> MELTPREKDKLLLFTAALVAERRLARGLKLNYPESVALISAFIMEGARDGKSVASLMEEGRHVLTREQVMEGVPEMI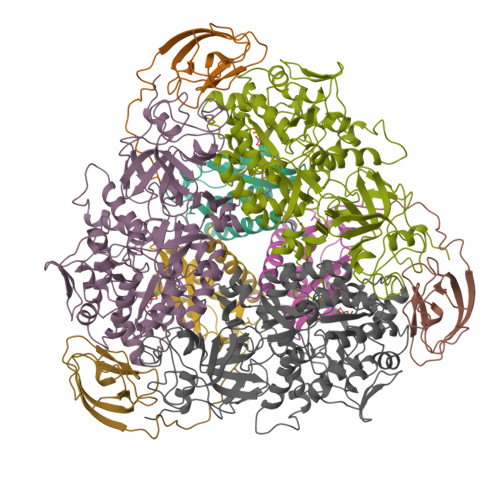PDIQVEATFPDGSKLVTVHNPII;> MIPGEYHVKPGQIALNTGRATCRVVVENHGDRPIQVGSHYHFAEVNPALKFDRQQAAGYRLNIPAGTAVRFEPGQKREVELVAFAGHRAVFGFRGEVMGPLEVNDE;> MSNISRQAYADMFGPTVGDKVRLADTELWIEVEDDLTTYGEEVKFGGGKVIRDGMGQGQMLAADCVDLVLTNALIVDHWGIVKADIGVKDGRIFAIGKAGNPDIQPNVTIPIGAATEVIAAEGKIVTAGGIDTHIHWICPQQAEEALVSGVTTMVGGGTGPAAGTHATTCTPGPWYISRMLQAADSLPVNIGLLGKGNVSQPDALREQVAAGVIGLKIHEDWGATPAAIDCALTVADEMDIQVALHSDTLNESGFVEDTLAAIGGRTIHTFHTEGAGGGHAPDIITACAHPNILPSSTNPTLPYTLNTIDEHLDMLMVAHHLDPDIAEDVAFAESRIRRETIAAEDVLHDLGAFSLTSSDSQAMGRVGEVILRTWQVAHRMKVQRGALAEETGDNDNFRVKRYIAKYTINPALTHGIAHEVGSIEVGKLADLVVWSPAFFGVKPATVIKGGMIAIAPMGDINASIPTPQPVHYRPMFGALGSARHHCRLTFLSQAAAANGVAERLNLRSAIAVVKGCRTVQKADMVHNSLQPNITVDAQTYEVRVDGELITSEPADVLPMAQRYFLF> TRKMWSVQESEWLKQGVVRYGVGHWERIRSAFPFAGRTAVNLKD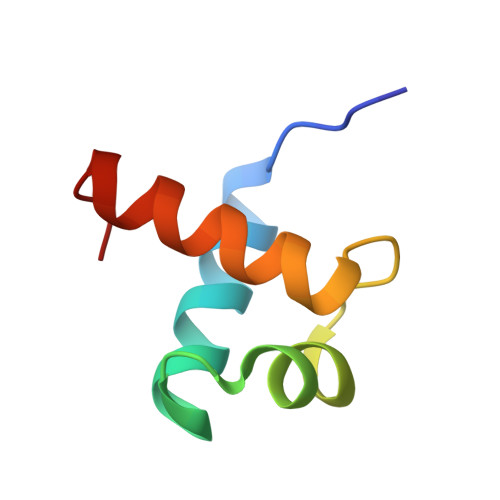RWRTMVKLKMV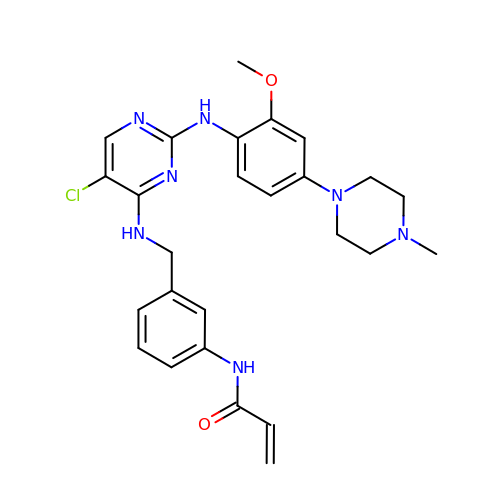N-(3-{[(5-chloro-2-{[2-methoxy-4-(4-methylpiperazin-1-yl)phenyl]amino}pyrimidin-4-yl)amino]methyl}phenyl)prop-2-enamide | C26 H30 Cl N7 O2 | UGXCBYVBIJACEK-UHFFFAOYSA-N> GSHMTRETERFPAREFQRDLLDWFARERRDLPWRKDRDPYKVWVSEVMLQQTRVETVIPYFEQFIDRFPTLEALADADEDEVLKAWEGLGYYSRVRNLHAAVKEVKTRYGGKVPDDPDEFSRLKGVGPYTVGAVLSLAYGVPEPAVDGNVMQVLSRLFLVTDDIAKPSTRKRFEQIVREIMAYENPGAFNEALIELGALVCTPRRPSCLLCPVQAYCQAFAEGVAEELPVKMKKTAVKQVPLAVAVLADDEGRVLIRKRDSTGLLANLWEFPSCETDGADGKEKLEQMVGEQYGLQVELTEPIVSFEHAFSHLVWQLTVFPGRLVHGGPVEEPYRLAPEDELKAYAFPVSHQRVWREYKEWASGVRPPP

MUTYH is a clinically important DNA glycosylase that thwarts mutations by initiating base-excision repair at 8-oxoguanine (OG):A lesions. Improperly placed adenines within pro-mutagenic OG:A base pairs are removed by the adenine glycosylase MUTYH, as the first step in Base Excision Repair (BER). The [4Fe-4S] cluster is coordinated by four cysteine ligands within the N-terminal catalytic domain, while the Zn(II) ion is coordinated by three cysteine ligands in the interdomain connector region (IDC) and one histidine within the catalytic domain. A loop made by two Cys residues that coordinate the [4Fe-4S] cluster, referred to as the iron-sulfur cluster loop, mediates electrostatic interactions with the DNA backbone that are critical for recognition of the lesion containing substrate.

In order to delineate the structural basis for the unexpected absence of activity for the R241Q MUTYH, we turned to the corresponding variant in Geobacillus stearothermophilus MutY (GsMutY), R149Q. R149Q is the analogous R241Q mutation in MUTYH. Of note, the Arg residue, and its participation in the H-bond network with the [4Fe-4S] cluster is highly conserved in MutY enzymes, and therefore likely plays a similar role. However, unlike the mutation in the human homolog, R149Q GsMutY retained measurable adenine glycosylase activity, but with a significant reduction on the base excision rate constant (k2) and turnover rate constant (k3) of ~50- and 5-fold relative to WT GsMutY, respectively. Alterations in the GsMutY structure in the immediate neighborhood of position 149 propagate to the [4Fe-4S] cluster and its Cys290 ligand to induce alternate conformations for the metal cofactor in the R149Q variant. Elongated features in the map calculated from anomalous differences clearly define two different conformations of the [4Fe-4S] cluster with a 1.4-Å displacement separating conformation A and conformation B, which refined with approximately equal group occupancies: q = 0.53 (A) and 0.47 (B). Another difference apparent for the R149Q GsMutY structure, is a calcium ion chelated by Oδ1 of Asn146. In the WT GsMutY structure, Oδ1 of Asn146 accepts an H-bond from Arg149. Apparently, loss of this Arg149-Asn146 H-bond creates an opportunity for invasion by divalent metal ions, such as Ca2+, which is abundantly present in the crystallization condition. Two structural states for the [4Fe-4S] cofactor, as revealed by these two variants, N146S and R149Q, in proximity to the active site and [4Fe-4S] cluster respectively, suggests that this allosteric network communicates events between the cofactor and active site for critical functional outcomes.> XKKKKKK;> XEYE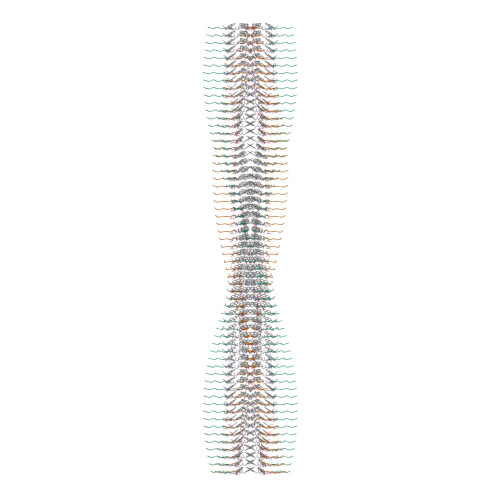YEY>[16x]ASWSHPQFEKIEGRRDRGPEFMAKQYKNLVNGEWKLSENEITIYAPATGEELGSVPAMTQAEVDAVYASAKKALSDWRTLSYVERAAYLHKAADILVRDAEKIGAILSKEVAKGHKAAVSEVIRTAEIINYAAEEGLRMEGEVLEGGSFEAASKKKIAIVRREPVGLVLAISPFNYPVNLAGSKIAPALIAGNVVALKPPTQGSISGLLLAEAFAEAGIPAGVFNTITGRGSVIGDYIVEHEAVNFINFTGSTPIGEGIGKLAGMRPIMLELGGKDSAIVLEDADLALAAKNIVAGAFGYSGQRSTAVKRVLVMDKVADQLAAEIKTLVEKLSVGMPEDDADITPLIDTSAADFVEGLIKDATDKGATALTAFNREGNLISPVLFDHVTTDMRLAWEEPFGPVLPIIRVTTVEEAIKISNESEYGLQASIFTTNFPKAFGIAEQLEVGTVHLNNKTQRGTDNFPFLGAKKSGAGVQGVKYSIEAMTTVKSVVFDIQ

GapN catalyzes the irreversible oxidation of glyceraldehyde 3-phosphate (G3P) to 3-phosphoglycerate (3-PG) while reducing NADP+ to NADPH. As S. pyogenes lacks the oxidative part of the pentose phosphate pathway, GapN appears to be the major NADPH source for the bacterium. The GapN-monomer from S. pyogenes, like its counterparts from other organisms can be subdivided into three domains (Cobessi et al., 1999). The monomers assemble into a tetramer displaying D2 symmetry which is formed by two interlacing dimers with dimer-dimer contacts primarily mediated by the protruding domain, while contacts within each dimer are formed by a β-sheet of the protruding domain interacting with a β-sheet of the catalytic α/β domain via salt bridges as well as α-helices (residues 232–251) of the Rossmannoid fold of each chain.

The structure revealed a covalent modification of the enzyme at the active site residue C284, which could be modeled as β-mercaptoethanol although this compound was not present during purification. Hence, the enzyme must have been modified following heterologous expression in E. coli. To eliminate this modification and generate a true apo-state of the enzyme, the C284S variant was generated and crystallized. Its crystal structure was also determined by molecular replacement, with a tetramer of the wild-type protein as search model. Due to its higher resolution, the structure of the C284S mutant is presented and discussed here. Starting at the N-terminus, residues 2–118, 145–252, and 450–464 form the cofactor binding domain containing a Rossmannoid fold (residues 145–252, cyan with the remainder of the domain in blue) which harbors five β-strands and three α-helices and mediates binding to NADP. The two other domains are the protruding domain composed of residues 119–144 and 464–475 (magenta), which is critical for oligomerization, and the catalytic α/β domain encompassing residues 253–445 (yellow). The catalytically active cysteine, which is responsible for the nucleophilic attack on the carbonyl carbon of G3P, is located at position 284, in close proximity to E250, the other key catalytic residue. In all chains of the wild-type and C284S variant a cis-peptide was observed while only half of the chains in the reference structure from S. mutans were modeled in the cis configuration. As this peptide bond is within 11.2 Å of the active site, it might be relevant for the proper function of the enzyme.methyl 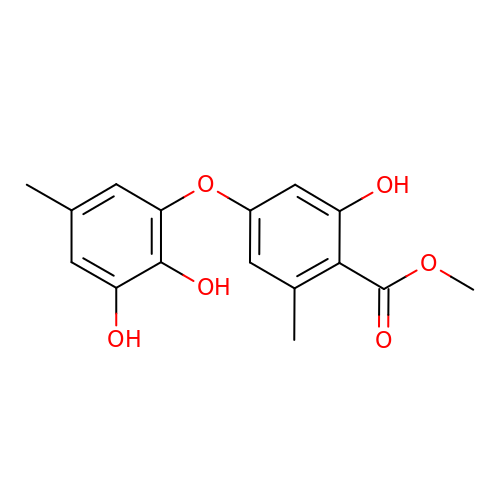4-(2,3-dihydroxy-5-methylphenoxy)-2-hydroxy-6-methylbenzoate | C16 H16 O6 | BLXSEOJIXHWXQJ-UHFFFAOYSA-N>[3x]MTTADLILINNWYVVAKVEDCRPGSITTAHLLGVKLVLWRSHEQNSPIQVWQDYCPHRGVPLSMGEVANNTLVCPYHGWRYNQAGKCVQIPAHPDMVPPASAQAKTYHCQERYGLVWVCLGNPVNDIPSFPEWDDPNYHKTYTKSYLIQASPFRVMDNSIDVSHFPFIHEGILGDRNHAEVEDLEVKVDKDGLTMGKYQVHTSKFNNSTKDDSMVNWFRLSHPLCQYCSTEASEMRTVDLMVVTPIDEDNSVLRYLIMWNGSKTLESKILADYDQVIEEDIRILHSQQPTRLPLLSPKQINTQGLPQEIHVPSDRCTVAYRRWLKELGVTYGVC

To investigate the architectural parameters that dictate the substrate specificity and site-selectivity of a Rieske oxygenase catalyzed reaction, we focused on two Rieske oxygenases, SxtT and GxtA, which are involved in the biosynthesis of paralytic shellfish toxins. These enzymes share 88% sequence identity with one another and selectively install a hydroxyl group on adjacent C12 and C11 positions of a tricyclic saxitoxin scaffold, respectively. Each structure showcases an α3 trimeric architecture, and each protomer of the trimer contains a Rieske cluster in the N-terminal domain and a non-heme iron center in the C-terminal domain. The trimeric quaternary architecture places these metallocenters within electron transfer distance of one another across the subunit-subunit interfaces.

Based upon the success of identifying a residue in the flexible loop that is involved in site selectivity, we experimentally probed the location of a substrate entrance tunnel to the active site. Crystals of SxtT and GxtA were pressurized with Xe, cryo-cooled, and placed in the X-ray beam. A resultant 2.69-Å resolution Xe-pressurized crystal structure of GxtA revealed the presence of Xe in each protomer of the trimeric architecture. The Xe binding sites were confirmed by calculation of anomalous maps. The Xe binding site is formed mainly by hydrophobic residues Val276, Leu173, Ile172, as well as Tyr273. In both proteins, the tunnels span a similar distance of approximately 33 Å. In particular, the GxtA tunnel showcases a higher hydropathy index than that of the tunnel found in SxtT and a larger bottleneck radius of 2.7 Å. This tunnel width is mainly limited by residues in the center of the tunnel (Thr230, Thr237, and Tyr273), whereas the smaller 1.7 Å tunnel radius observed in SxtT is limited by residues located near the entrance (Ser230, Ile237, and Glu272).>MVRLGPKKPPARKGSMADVPANLMEQIHGLETLFTVSSEKMRSIVKHFISELDKGLSKKGGNIPMIPGWVVEYPTGKETGDFLALDLGGTNLRVVLVKLGGNHDFDTTQNKYRLPDHLRTGTSEQLWSFIAKCLKEFVDEWYPDGVSEPLPLGFTFSYPASQKKINSGVLQRWTKGFDIEGVEGHDVVPMLQEQIEKLNIPINVVALINDTTGTLVASLYTDPQTKMGIIIGTGVNGAYYDVVSGIEKLEGLLPEDIGPDSPMAINCEYGSFDNEHLVLPRTKYDVIIDEESPRPGQQAFEKMTSGYYLGEIMRLVLLDLYDSGFIFKDQDISKLKEAYVMDTSYPSKIEDDPFENLEDTDDLFKTNLNIETTVVERKLIRKLAELVGTRAARLTVCGVSAICDKRGYKTAHIAADGSVFNRYPGYKEKAAQAL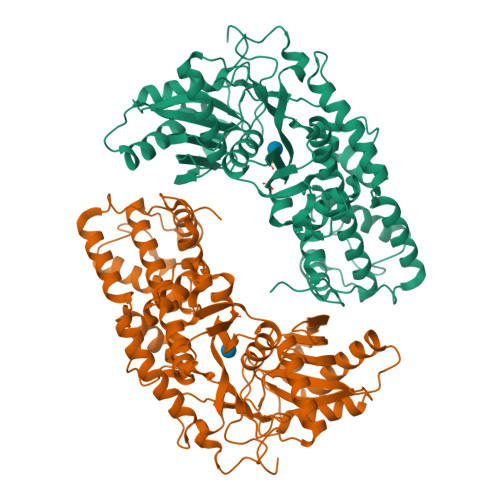KDIYNWDVEKMEDHPIQLVAAEDGSGVGAAIIACLTQKRLAAGKSVGIKGE[2x]> GGAUCGCUGAACCCGAAAGGGGCGGGGGACCCAGAAAU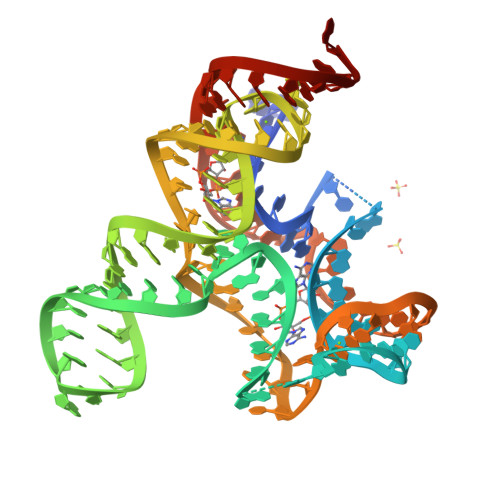GGGGCGAAUCUCUUCCGAAAGGAAGAGUAGGGUUACUCCUUCGACCCGAGCCCGUCAGCUAACCUCGCAAGCGUCCGAAGGAGAAUC>MAQAKHKQRKRLKSSCKRHPLYVDFSDVGWNDWIVAPPGYHAFYCHGECPFPLADHLNSTNHAIVQTLVNSVNSKIPKACCVPTELSAISMLYLDENEKVVLKNYQDMVVEGCGCR[2x];>[2x]GSGAMAQNLDSMLHGTGMKSDSDQKKSENGVTLAPEDTLPFLKCYCSGHCPDDAINNTCITNGHCFAIIEEDDQGETTLASGCMK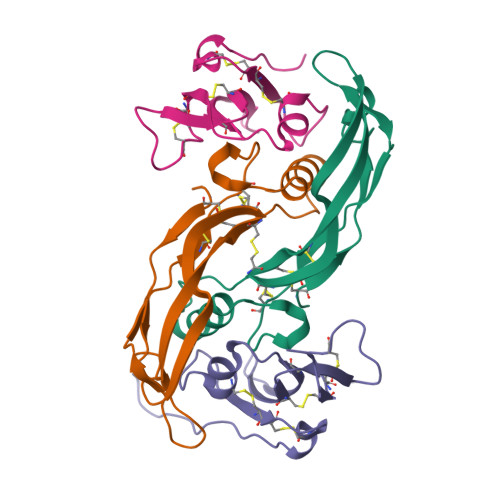YEGSDFQCRDTPIPHQRRSIECCRTNLCNQYLQPTLPPVVIGPFFDGSIR> TGGVQTVTLIPGDGIGPEISAAVMKIFDAAKAPIQWEERNVTAIQGPGGKWMIPSEAKESMDKNKMGLKGPLKTPIAAGHPSMNLLLRKTFDLYANVRPCVSIEGYKTPYTDVNIVTIRENTEGEYSGIEHVIVDGVVQSIKLITEGASKRIAEFAFEYARNNHRSNVTAVHKANIMRMSDGLFLQKCREVAESCKDIKFNEMYLDTVCLNMVQDPSQFDVLVMPNLYGDILSDLCAGLIGGLGVTPSGNIGANGVAIFESVHGTAPDIAGKDMANPTALLLSAVMMLRHMGLFDHAARIEAACFATIKDGKSLTKDLGGNAKCSDFTEEICRRVKDLD;> FSEQTIPPSAKYGGRHTVTMIPGDGIGPELMLHVKSVFRHACVPVDFEEVHVSSNADEEDIRNAIMAIRRNRVALKGNIETNHNLPPSHKSRNNILRTSLDLYANVIHCKSLPGVVTRHKDIDILIVRENTEGEYSSLEHESVAGVVESLAIITKAKSLRIAEYAFKLAQESGRKKVTAVHKANIMKLGDGLFLQCCREVAARYPQITFENMIVDNTTMQLVSRPQQFDVMVMPNLYGNIVNNVCAGLVGGPGLVAGANYGHVYAVFETATRNTGKSIANKNIANPTATLLASCMMLDHLKLHSYATSIRKAVLASMDNENMHTPDIGGQGTTSEAIQDVIRHIRVINGRAVEA

Isocitrate dehydrogenases (IDHs) are a family of enzymes that catalyze the oxidative decarboxylation of isocitrate (ICT) into α-ketoglutarate (α-KG) using NADP or NAD as coenzyme. The α and β subunits form one heterodimer (αβ) and the α and γ subunits form another heterodimer (αγ), which are assembled into a heterotetramer (α2βγ) and further into a heterooctamer (the heterotetramer and heterooctamer are sometimes called holoenzyme). Our biochemical data demonstrate that the αγ heterodimer exhibits similar enzymatic properties as the α2βγ heterotetramer and can be positively regulated by CIT and ADP, whereas the αβ heterodimer has only basal activity and cannot be regulated. The active site is located in the cleft formed by the large and small domains of the α subunit and the small domain of the γ subunit, and comprises of the binding sites for the metal ion, substrate ICT and coenzyme NAD.

To investigate the structural basis for the functional roles of these residues in the allosteric regulation, we took the γ-K151A mutation as a representative and determined the crystal structure of the αγK151A mutant bound with Mg2+, CIT and ADP at the allosteric site. In the αγK151AMg+CIT+ADP structure, the structure of the allosteric site is very similar to that in the αMgγMg+CIT+ADP structure with the CIT, ADP and Mg2+ binding to the allosteric site in similar manners and maintaining almost identical interactions. In addition, accompanying with the conformational changes of Arg97G and Tyr135G, the N-terminal part of the β5G–β6G loop and the N-terminal region of the α7G helix at the heterodimer interface also undergo similar conformational changes as in the αMgγMg+CIT+ADP structure. However, the C-terminal part of the β5G–β6G loop and the β7G strand assume similar conformations as in the αMgγ structure. Specifically, the hydrogen bond between the main-chain amine of Glu134G and the main-chain carbonyl of Asn235G is disrupted and the side chain of Glu134G is inserted into the space formerly occupied by the N-terminal loop of the α7G helix and forms a hydrogen bond with the main-chain amine of Leu236G. Due to the γ-K151A mutation, the hydrogen-bonding interactions of Lys151G with Asp190G and Tyr237G are lost but the hydrogen bond between the main-chain amine of Leu138G and the main-chain carbonyl of Leu150G is maintained. As a result, the β7G strand has no conformational change, and consequently the β7A strand, the β5A–β6A loop and the N-terminal region of the α7A helix also have no conformational changes and adopt similar conformations as in the αMgγ structure.1-[(3-CYCLOHEXYLPROPANOYL)(2-HYDROXYETHYL)AMINO]-1-DEOXY-D-ALLITOL 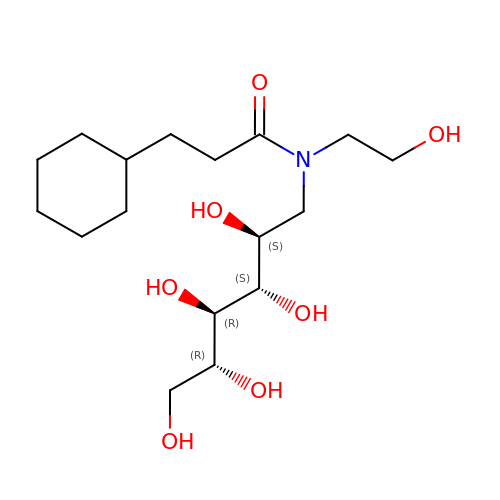| C17 H33 N O7 | AHJZPLOICPCLQM-HDEZJCGLSA-N Our model protein for comparing methods of RT structure determination is the coelomic hemoglobin from the marine annelid Amphitrite ornata. Named dehaloperoxidase (DHP; Chen et al., 1996; Zhang et al., 1996), this O2-transport protein is capable of oxidizing a wide array of substrates by either electron or O-atom transfer. DHP exhibits four activities common to heme proteins, peroxidase, peroxy­gen­ase, oxidase and oxygenase, with each activity employing an Fe(IV)-oxo (ferryl) intermediate. In this study, structures of a multifunctional globin, dehaloperoxidase B (DHP-B), obtained using several methods of room-temperature crystallographic structure determination are described and compared.

In this structure, the heme iron is pentacoordinate in both protomers, with no evidence of a distal water or dioxygen ligand. There is no electron density to indicate a hemichrome species in protomer A in this case. Notably, in both protomers the distal His55 residue is swung away from the heme iron and towards the protein surface [Fig. 2(c)]. A water molecule has been modelled in the distal pocket of protomer B. Due to its position, this density could also arise from the alternate swung-in conformer of His55, particularly since a water molecule at this position would not be stabilized by hydrogen bonding to any protein residue or heme propionate. In our SLX data, difference density indicates a weak area of positive electron density suggesting a dual conformation of His55 (data not shown). Modelling of a dual conformation for this residue did not prove stable in refinement and so only the primary conformation was included in the final model. The observation of conformational change of His55 in the ‘swung-out’ position, in contrast to its ‘swung-in’ conformation in the damage-free structures (SFX and NX), implies another site-specific radiation-damage effect. A major advantage of the Laue method is that far fewer (181) crystals were required for the Laue approach than for the other microcrystal-based approaches, with the drawback of more challenging data processing. SLX is particularly valuable where limited numbers of microcrystals are available, requiring far fewer crystals than are needed for either SSX or SFX.

>[2x]MGFKQDIATLRGDLRTYAQDIFLAFLNKYPDEKRNFKNYVGKSDQELKSMAKFGDHTEKVFNLMMEVADRATDCVPLASDASTLVQMKQHSGLTTGNFEKLFVALVEYMRASGQSFDSQSWDRFGKNLVSALSSAGMK> PISPIETVPVKLKPGMDGPKVKQWPLTEEKIKALVEICTEMEKEGKISKIGPENPYNTPVFAIKKKD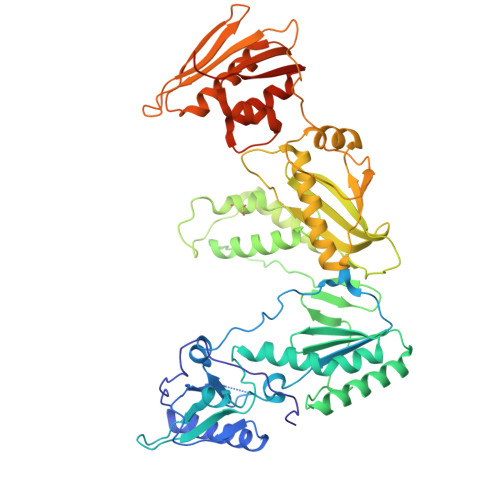STKWRKLVDFRELNKRTQDFWEVQLGIPHPAGIKKKKSVTVLDVGDAYFSVPLDEDFRKYTAFTIPSINNETPGIRYQYNVLPQGWKGSPAIFQSSMTKILEPFRKQNPDIVIYQYMDDLYVGSDLEIGQHRTKIEELRQHLLRWGLTTPDKKHQKEPPFLWMGYELHPDKWTVQPIVLPEKDSWTVNDIQKLVGKLNWASQIYPGIKVRQLCKLLRGTKALTEVIPLTEEAELELAENREILKEPVHGVYYDPSKDLIAEIQKQGQGQWTYQIYQEPFKNLKTGKYARMRGAHTNDVKQLTEAVQKITTESIVIWGKTPKFKLPIQKETWETWWTEYWQATWIPEWEFVNTPPLVKLWYQLEKEPIVGAETFYVDGAANRETKLGKAGYVTNRGRQKVVTLTDTTNQKTELQAIYLALQDSGLEVNIVTDSQYALGIIQAQPDQSESELVNQIIEQLIKKEKVYLAWVPAHKGIGGNEQVDKLVSAGIRKVL>[2x]MPDMANVESFDLDHTKVKAPYVRLAGVKTTPKGDQISKYDLRFLQPNQGAIDPAAIHTLEHL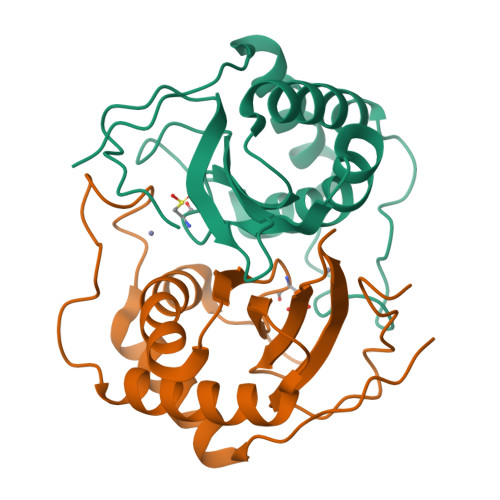LAGYMRDHLEGVVDVSPMGCRTGMYMAVIGEPDEQGVMKAFEAALKDTAGHDQPIPGVSELECGNYRDHDLAAARQHARDVLDQGLKVQETILLERGSHHHHHH> MSLPLLRPFETVSLENAVEDLVVRFILNVPPEDLSTVERVLFHFEEASWFYTDFVKLMNPYLPNLSIKSFSKIVIDICPLIWNWDITPENALVKFSNYKKTIPVRGAAIFNDSLSKILLLRGINSKHWSFPRGKIGKDEDDVACCIREVKEETGFDLTGFIDADQYVERNM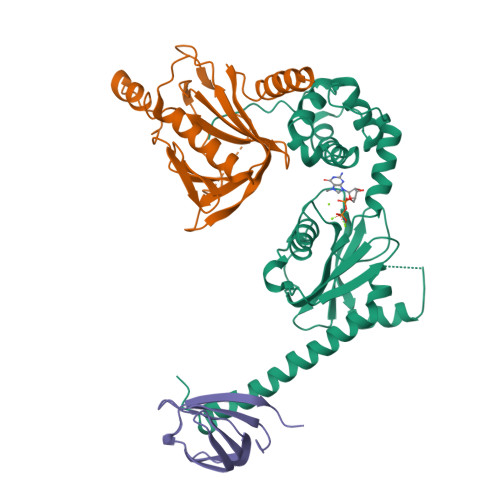NGKNFKIFLVKGVPEDFEFKPEHKNEIQAIEWKDFKKLSKAITKNEGSAKVFLVNSMIRPLSLYVKNEKRAKDENKLKLYAEEHLKSILGLNKKENKIVLDAGRHHHHHH;> MSTETLEIYRKALNFNVIARYDPKIKQLLFHTPHATVYKWGDDNWNKLEYQGVLAIYLRDVGDKEAILPEVSSYDDTITGQQSEANTPHVLTGHDIYNYGLIIMNRINPDNFSLAIAPNSVLNKRKLFAPNREEELEPMKVEVRDDLVMIKTLKKEVYGIWVHTPEDRQNIYELIKYLLENEPTDSFT;> MLNFKGYQIEIELKDGKRITGTLKQVSPKSLTLTDAVFQDGGVSPVFKIKADKLYDLKVLKLPPNA> MPTLFDPIDFGPIHAKNRIVMSPLTRGRADKEAVPTPIMAEYYAQRASAGLIITEATGISREGLGWPFAPGIWSDAQVEAWKPIVAGVHAKGGKIVCQLWHMGRMVHSSVTGTQPVSSSATTAPGEVHTYEGKKPFEQARAIDAADISRILNDYENAARNAIRAGFDGVQIHAANGYLIDEFLRNGTNHRTDEYGGVPENRIRFLKEVTERVIAAIGADRTGVRLSPNGDTQGCIDSAPETVFVPAAKLLQDLGVAWLELREPGPNGTFGKTDQPKLSPQIRKVFLRPLVLNQDYTFEAAQTALAEGKADAI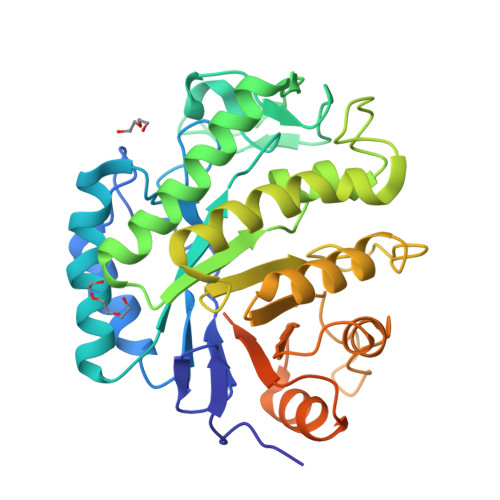AFGRKFISNPDLPERFARGIALQPDDMKTWYSQGPEGYTDYPSATSGPN>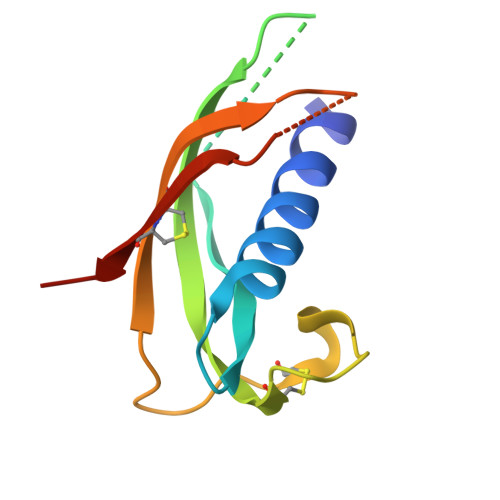 QALSYREAVLRAVDRLNEQSSEANLYRLLELDQPPKADEDPGTPKPVSFTVKETVCPRPTRQPPELCDFKENGRVKQCVGTVTLDQIKDPLDITCNEVQGV>[2x]IDFSLTEEQRQLQALARRFAKEVILPVAQEYDEKEEVPWPVIEKLHEVGLLNAIIPEEYGGMGLKMLDEVIVGEELAYACMGIYTIPMASDLGITPVLLAGTEEQKERFLRPLTEKPALAAFALSEPGNGSDAAALKTRAIRQGDH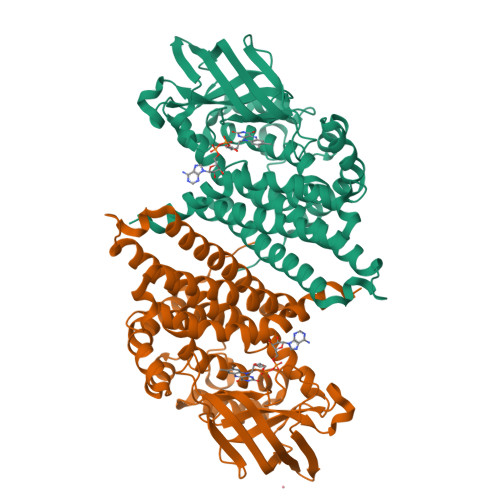YVLNGTKMWISNGGEAEWVVVFATVNPELRHKGVVALVVERGTPGFKAIKIHGKMGQRASGTYELVFEDVKVPVENRLGEEGEGFKIAMQTLNKTRIPVAAGSVGVARRALDEARKYAKEREAFGEPIANFQAIQFKLVDMLIGIETARMYTYYAAWLADQGLPHAHASAIAKAYASEIAFEAANQAIQIHGGYGYVREFPVEKLLRDVKLNQIYEGTNEIQRLIIARHILAA> MRRRAVLGGAVVYPEGPPPSYESVMQQQAAMIQPPLEAPFVPPRYLAPTEGRNSIRYSELSPLYDTTKLYLVDNKSADIASLNYQNDHSNFLTTVVQNNDFTPTEASTQTINFDERSRWGGQLKTIMHTNMPNVNEYMFSNKFKARVMVSRKAPEGVTVNDTYDHKEDILKYEWFEFILPEGNFSATMTIDLMNNAIIDNYLEIGRQNGVLESDIGVKFDTRNFRLGWDPETKLIMPGVYTYEAFHPDIVLLPGCGVDFTESRLSNLLGIRKRHPFQEGFKIMYEDLEGGNIPALLDVTAYEESKKDTTTETTTKKELKIQPLEKDSKSRSYNVLEDKINTAYRSWYLSYNYGNPEKGIRSWTLLTTSDVTCGAEQVYWSLPDMMQDPVTFRSTRQVNNYPVVGAELM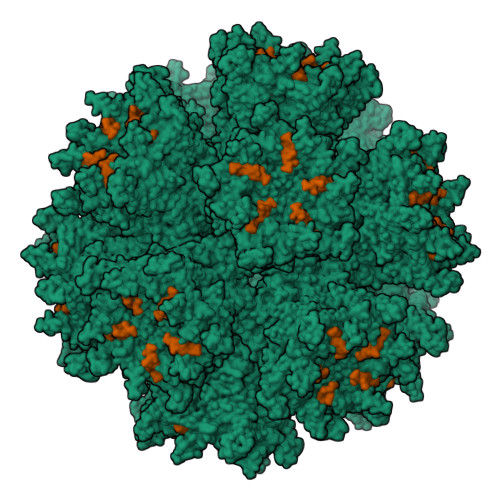PVFSKSFYNEQAVYSQQLRQATSLTHVFNRFPENQILIRPPAPTITTVSENVPALTDHGTLPLRSSIRGVQRVTVTDARRRTCPYVYKALGIVAPRVLSSR;> MKRARPSEDTFNPVYPYDTEC>[2x]SFKAAGTSGLILKRCSEPERYCLARLMADALRGCVPAFHGVVERDGESYLQLQDLLDGFDGPCVLDCKMGVRTYLEEELTKARERPKLRKDMYKKMLAVDPEAPTEEEHAQRAVTKPRYMQWREGISSSTTLGFRIEGIKKADGSCSTDFKTTRSREQVLRVFEEFVQGDEEVLRRYLNRLQQIRDTLEVSEFFRRHEVIGS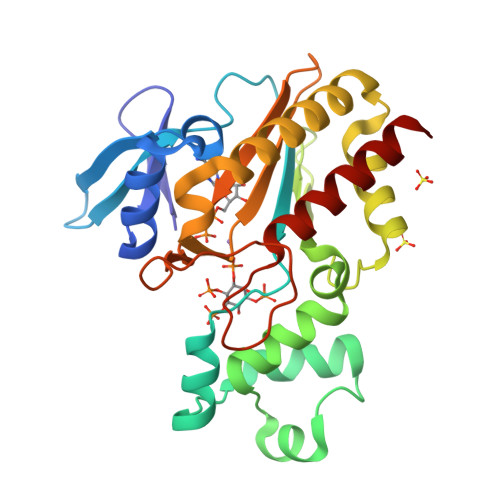SLLFVHDHCHRAGVWLIDFGKTTPLPDGQILDHRRPWEEGNREDGYLLGLDNLIGILASLAER> MESRKLISATDIQYSGSLLNSLNEQRGHGLFCDVTVIVEDRKFRAHKNILSASSTYFHQLFSVAGQVVELSFIRAE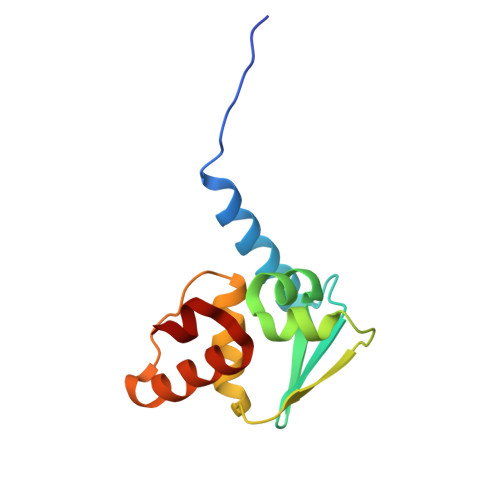IFAEILNYIYSSKIVRVRSDLLDELIKSGQLLGVKFIAAL> ECCTSRELVEFKMDRGDCEAVRAIENYPNGCEVTICADG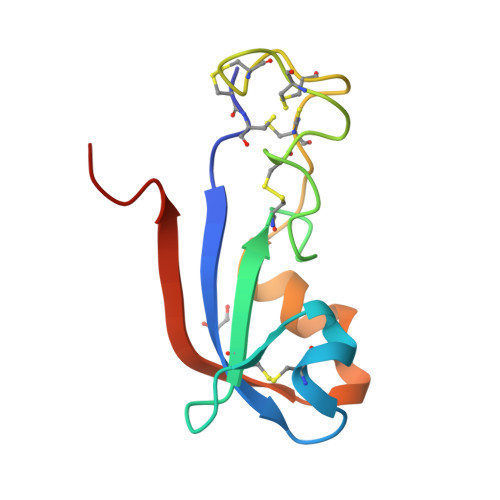VAQLGAYCGQGPCNIFGCNCDGGCLSGDWSQEFVRRNQQYGIQIIKVTRLPFWRPL N-[(2Z)-4-(3-fluoro-5-morpholin-4-ylphenyl)pyrimidin-2(1H)-ylidene]-4-(3-morpholin-4-yl-1H-1,2,4-triazol-1-yl)aniline 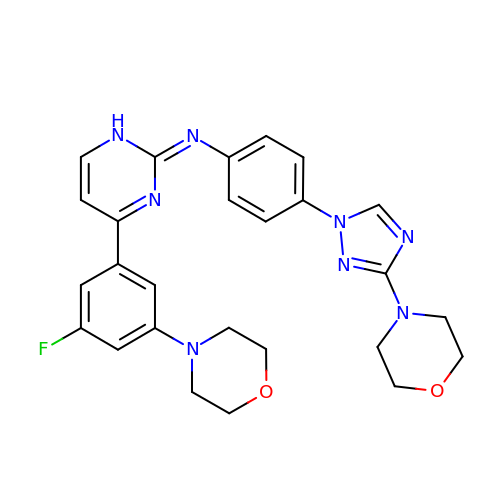| C26 H27 F N8 O2 | AHMHIFXJPSHHPH-UHFFFAOYSA-N>[2x]GSHMHTLYAPGGYDIMGYLIQIMNRPNPQVELGPVDTSCALVLCDLKQKDTPVVYASEAFLYMTGYSNAEVLGRNCRFLQSPDGMVKPKSTRKY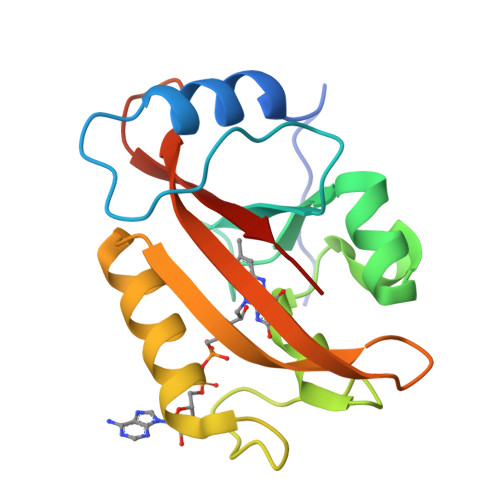VDSNTINTMRKAIDRNAEVQVEVVNFKKNGQRFVNFLTMIPVRDETGEYRYSMGFQCETE>[2x]HHHHHHSSGLVPRGSMDIRALYDEKLTTPEEAVSSIASGSHLSMGMFAAEPPALLKALADRATRGDIGDLRVYYFETAKIAGDTILRYELNNRIK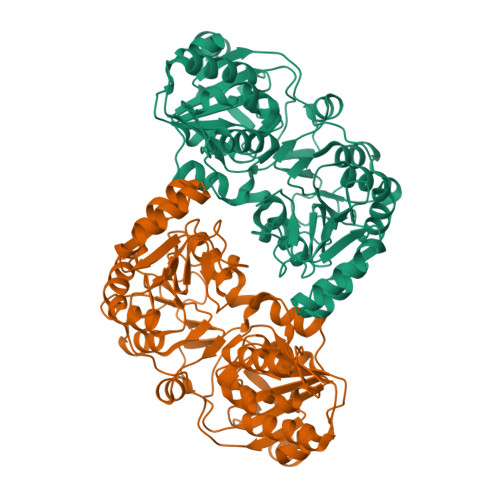PYSMFVTAVERALIRRGIEDGGRKVVNYVPSNFHQAPRLLAEEIGIDTFMHTVSPMDCHGYFSLGVGNDYSSRIARSARRFIVEVNRYMPRVQGEAAAIHISEVDAIVENHVPLIEMPVRSAIPEYTSISHIIADLVPDGACLQMGVGALPNLVCGVLKDRNDLGIHTEVLNPGLVDLIRRGVVTNQRKTLDRGRSVFTFAMGQQEMYEYLNDHPAIFSRPVDYVNDPHIIAQNDNVVSINATLQIDLTGACNSEHMLGHQYSASGGQLDFVRGAYASKGGRSIIATPSTAAKGTVSRIIPRIDGPVTTPRIDTHYIVTEFGAVNLKGLSSTERALRIIELAHPDFRDELTQAAKKMHLI>[4x]GMIDTFERTGPLMEASSYPAWAQQLINDCSPAKARVVEHELYQQMRDAKLSPQIMRQYLIGGWPVVEQFAVYMAKNLTKTRFGRHPGEDMARRWLMRNIRVELNHADYWVNWCAAHDVTLEDL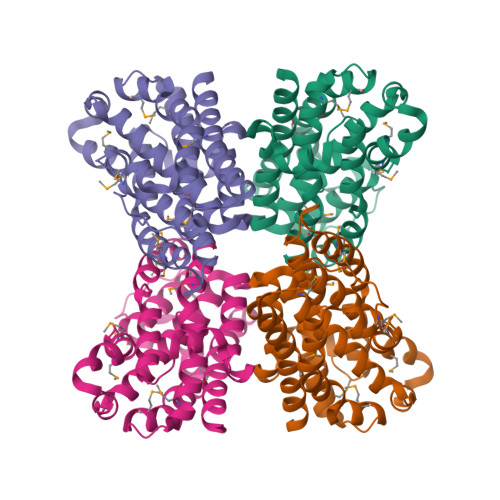HDQRVAPELHALSHWCWQTSSSDSLAVAMAATNYAIEGATGEWSAVVCSTGVYAEAFAEETRKKSMKWLKMHAQYDDAHPWEALEIICTLVGNKPSLQLQAELRQAVTKSYDYMYLFLERCIQLDKVKSPRGRVAALEM>MSNEYDEYIANHTDPVKAINWNVIPDEKDLEVWDRLTGNFWLPEKIPVSNDIQSWNKMTPQEQLATMRVFTGLTLLDTIQGTVGAISLLPDAETMHEEAVYTNIAFMESVHAKSYSNIFMTLASTPQINEAFRWSEENENLQRKAKI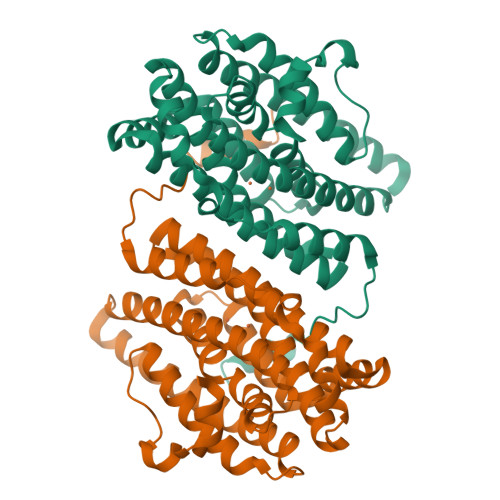IMSYYNGDDPLKKKVASTLLESFLFYSGFYLPMYLSSRAKLTNTADIIRLIIRDESVHGYYIGYKYQQGVKKLSEAEQEEYKAYTFDLMYDLYENEIEYTEDIYDDLGWTEDVKRFLRYNANKALNNLGYEGLFPTDETKVSPAILSSLSPNADENHDFFSGSGSSYVIGKAEDTTDDDWDF[2x]> SLSLVDASWELVDPTPDLQALFVQFNDQFFWGQLEAVEVKW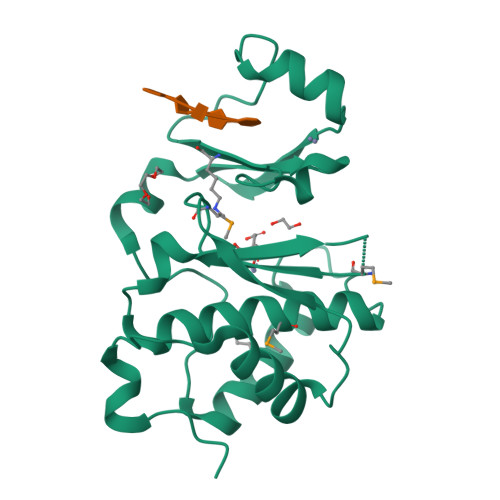SVRMTLCAGICSYEGKMCSIRLSEPLLKLRPRKDLVETLLHEMIHAYLFVTNNDKDREGHGPEFCKHMHRINSLTGANITVYHTFHDEVDEYRRHWWRCNGPCQHRPPYYGYVKRATNREPSAHDYWWAEHQKTCGGTYIKIKE>[2x]MVNSDSHPLFVRSLAKNMTWQLADTSTQKVLASGASATSGDK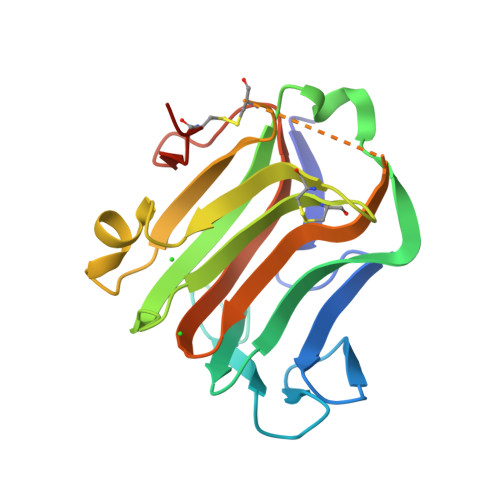QSLLMQSVNLSYQEDGRGFNWRAQAALSLSYLEPTPLDSKFSTGYLELKMRIDKAPEQGANLQVMCSESNCLRDIDFSSFSQLMADKSWHTLAIPLHCDDSDQAEQPITDALRITSQNLSLAIADVALTIKPSDDSISLTCAKLEHHHHHH> MHHHHHHDADYPLRVLYCGVCSLPTE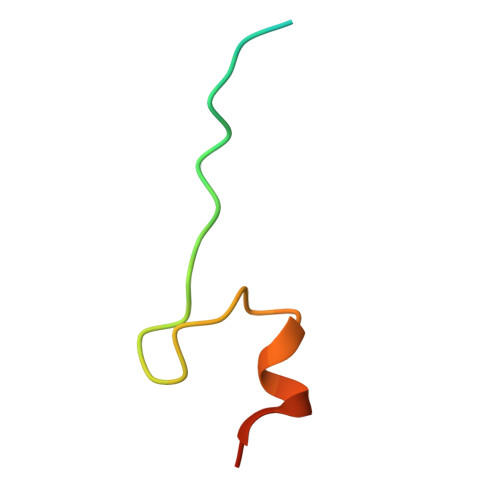YCEYMPDVA>GSHMGVTVERIAPGDGKNFPKKGDKVTIHYVGTLENGDKFDSSRDRGSPFQCTIGVGQVIKGWDEGVTQLSVGEKARLICTHDYAYGER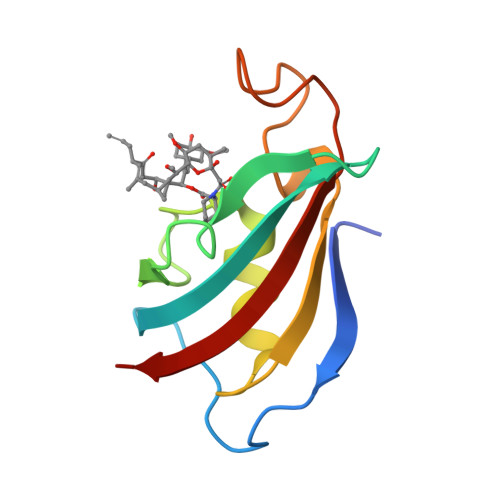GYPGLIPPKATLNFEVELIKIN[4x]>MARLEDPTALTQLPDESARVRYTSSELQDYFETLKFPQRFLDLGNSVLKDPSLARTKENGLPLLQAITRYHTCNVPFENLVLHYDPHKIVTLDPAELYTKIVTRRRGGRCMENNIFLGTALRSLGYEVRNCGGRVSRAMSPYPEVRKNQSATYDGWNHMLLLVFLGDEWYGVDVGMGSMGPNLPFPLQDGFESLSIAPREIRIQKRSISETHATGPSHATKMWCYDVCYNPAESKKTWTPVYCFTETEFLPQDYEVMSWFTSTNPRSFFTRYITCTKMIMDEDKEVIIGNLTLFKDTVRETIGSDRKVVKKFETEEERIKG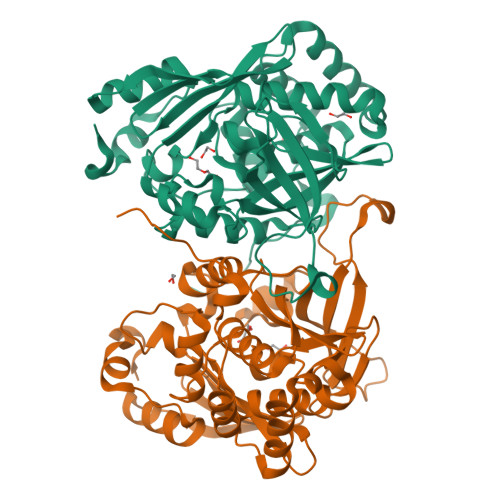LVEIFDVNLTEEEKNSLPQEKRL[4x]>[2x]HPPSYVAHLASDFGVRVFQQVAQASKDRNVVFSPYG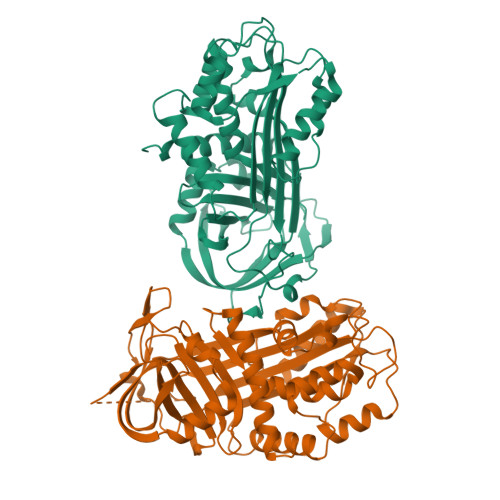VASVLAMLQLTTGGETQQQIQAAMGFKIDDKGMAPALRHLYKELMGPWNKDEISTTDAIFVQRDLKLVQGFMPHFFRLFRSTVKQVDFSEVERARFIINDWVKTHTKGMISHLLGTGAVDQLTRLVLVNALYFNGQWKTPFPDSSTHRRLFHKSDGSTVSVPMMAQTNKFNYTEFTTPDGHYYDILELPYHGDTLSMFIAAPYEKEVPLSALTNILSAQLISHWKGNMTRLPRLLVLPKFSLETEVDLRKPLENLGMTDMFRPFQADFTSLSDQEPLHVALALQKVKIEVNESGTVASSSTAVIVSARMAPEEIIIDRPFLFVVRHNPTGTVLFMGQVMEP> DVPVNLYRPNAPFIGKVISNEPLVKEGGIGIVQHIKFDLTGGNLKYIEGQSIGIIPPGVDKNGKPEKLRLYSIASTRHGDDVDDKTISLCVRQLEYKHPESGETVYGVCSTYLTHIEPGSEVKITGPVGKEMLLPDDPEANVIMLATGTGIAPMRTYLWRMFKDAERAANPEYQFKGFSWLVFGVPTTPNILYKEELEEIQQKYPDNFRLTYAISREQKNPQG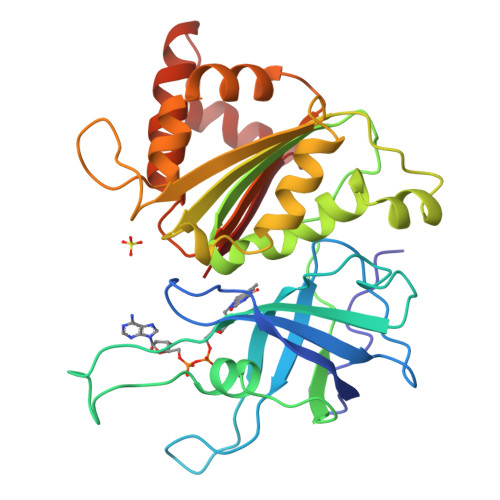GRMYIQDRVAEHADQLWQLIKNQKTHTYICGLEGMEEGIDAALSAAAAKEGVTWSDYQKDLKKAGRWHVETY D-XYLITOL-5-PHOSPHATE | C5 H13 O8 P | 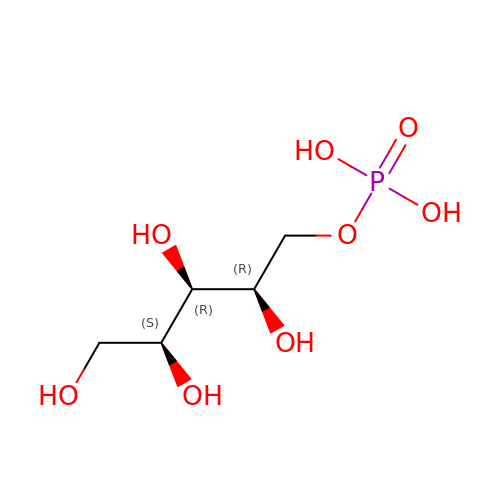VJDOAZKNBQCAGE-VPENINKCSA-N> MKIRSQVGMVLNLDKAIGCHTCSVTCKNVWTSREGVEYAWFNNVETKPGQGFPTDWENQEKYKGGWIRKINGKLQPRMGNRAMLLGKIFANPHLPGIDDYYEPFDFDYQNLHTAPEGSKSQPIARPRSLITGERMAKIEKGPNWEDDLGGEFDKLAKDKNFDNIQKAMYSQFENTFMMYLPRLCEHCLNPACVATCPSGAIYKREEDGIVLIDQDKCRGWRMCITGCPYKKIYFNWKSGKSEKCIFCYPRIEAGQPTVCSETCVGRIRYLGVLLYDADAIERAASTENEKDLYQRQLDVFLDPNDPKVIEQAIKDGIPLSVIEAAQQSPVYKMAMEWKLALPLHPEYRTLPMVWYVPPLSPIQSAADAGELGSNGILPDVESLRIPVQYLANLLTAGDTKPVLRALKRMLAMRHYKRAETVDGK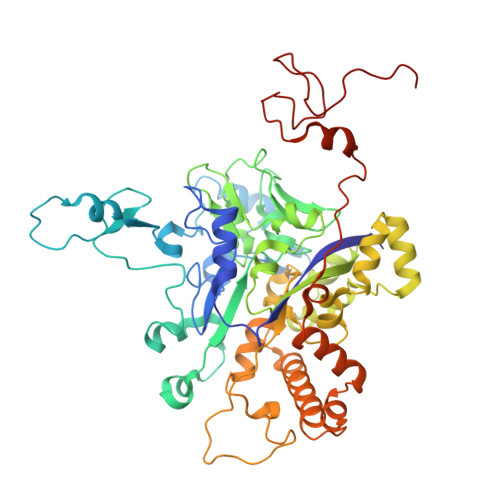VDTRALEEVGLTEAQAQEMYRYLAIANYEDRFVVPSSHRELAREAFPEKNGCGFTFGDGCHGSDTKFNLFNSRRIDAIDVTSKTE4-methyl-~{N}-[(1~{R})-1-phenylethyl]piperidine-1-carboxamide | C15 H22 N2 O | 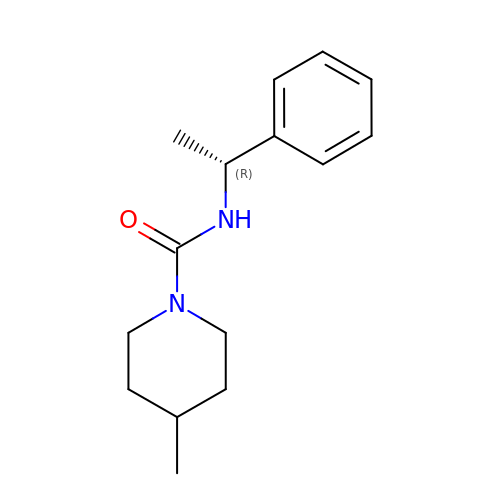PSSJJOIQPKCPGY-CYBMUJFWSA-N> ANFL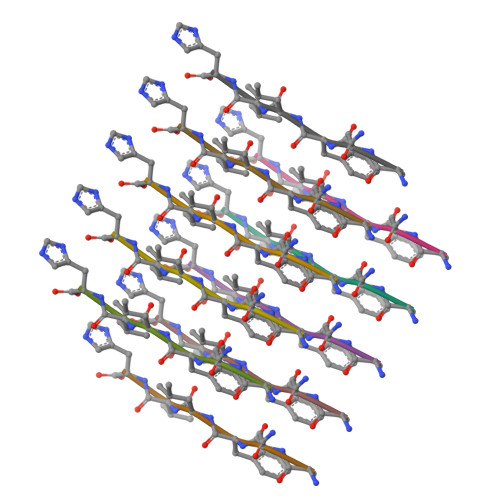VH>[6x]GSMGRPALYFCGSIRGGREDRT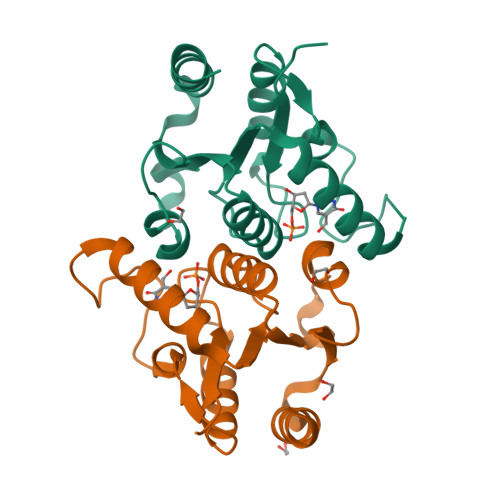LYERIVSRLRRFGTVLTEHVAAAELGARGEEAAGGDRLIHEQDLEWLQQADVVVAEVTQPSLGVGYQLGRAVAFNKRILCLFRPQSGRVLSAMIRGAADGSRFQVWDYEEGEVEALLDRYFEADP> MSLSNKLTLDKLDVKGKRVVMRVDFNVPMKNNQITNNQRIKAAVPSIKFCLDNGAKSVVLMSHLGRPDGVPMPDKYSLEPVAVELKSLLGKDVLFLKDCVGPEVEKACANPAAGSVILLENLRFHVEEEGKGKDASGNKVKAEPAKIEAFRASLSKLGDVYVNDAFGTAHRAHSSMVGVNLPQKAGGFLM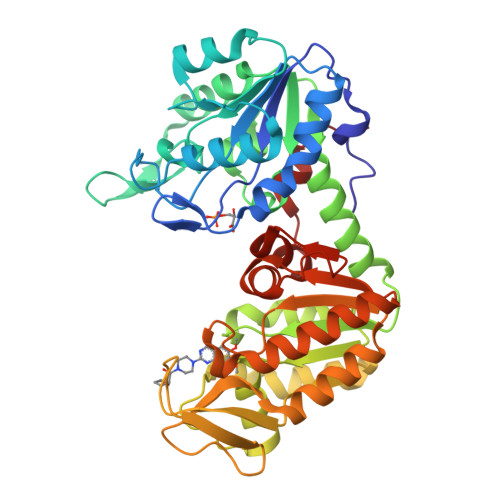KKELNYFAKALESPERPFLAILGGAKVADKIQLINNMLDKVNEMIIGGGMAFTFLKVLNNMEIGTSLFDEEGAKIVKDLMSKAEKNGVKITLPVDFVTADKFDENAKTGQATVASGIPAGWMGLDCGPESSKKYAEAVTRAKQIVWNGPVGVFEWEAFARGTKALMDEVVKATSRGCITTIGGGDTATCCAKWNTEDKVSHVSTGGGASLELLEGKVLPGVDALSNI>[2x]MQPWGRLLRLG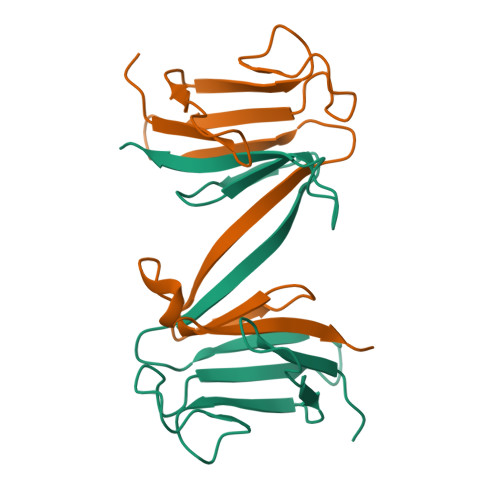AEEGEPHVLLRKREWTIGRRRGCDLSFPSNKLVSGDHCRIVVDEKSGQVTLEDTSTSGTVINKLKVVKKQTCPLQTGDVIYLVYRKNEPEHNVAYLYESLS>MRYRPFGSTGVAVSALTLRLADNPRLRANDWRALVFTALENGVNSFQIDGDAPELLKGAGEAFASVERHLLFLTWRLRGDAKQLGPHTLDALKRSAFEGLSLDYLDLLLINDPQSASLPMAFESGLQDLQKGRALRGLGVASRGDIDPGLLANDLVTAVSSPYNLSSGWAERHRIRQASQNNFAVIGEDFWPQALRELADVGGYEFLTNTPGWSAEDICLGYALTEPSLATVRVTADNRQEIERLAAVVERDLPTGVCAQIEMARFSAQER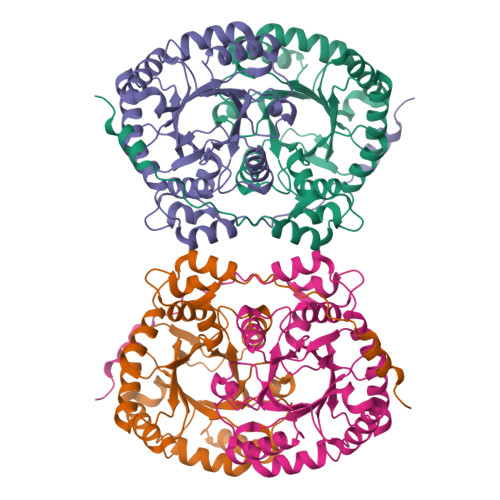EKAARRPKLAAALEHHHHEK[4x]> VDISTLPRVKVDLVKPPFVHAHDQVAKTGPRVVEFTMTIEEKKLVIDREGTEIHAMTFNGSVPGPLMVVHENDYVELRLINPDTNTLLHNIDFHAATGALGGGALTQVNPGEETTLRFKATKPGVFVYHCAPEGMVPWHVTSGMNGAIMVLPRDGLKDEKGQPLTYDKIYYVGEQDFYVPKDEAGNYKKYETPGEAYEDAVKAMRTLTPTHIVFNGAVGALTGDHALTAAVGERVLVVHSQANRDTRPHLIGGHGDYVWATGKFRNPPDLDQETWLIPGGTAGAAFYTFRQPGVYAYVNHNLIEAFELGAAGHFKVTGEWNDDLMTSVVKPASM

Copper nitrite reductases (CuNiRs) found in fungi, bacteria and archaea belong to a highly conserved enzyme family that catalyze the one-electron reduction of nitrite to NO [NO2− + e− + 2H+ ⇆ NO + H2O]. The involvement of CuNiRs in two branches of the global nitrogen cycle, denitrification and nitrification, make them of critical environmental importance since N2O is a major by-product of denitrification, which is the third most significant greenhouse gas with a global warming potential 300 times that of CO2.3 The catalytic type 2 Cu centre (T2Cu) of CuNiR is located at the interface of two adjacent monomers and linked to the electron-donating T1Cu centre via a Cys–His bridge. Two invariant active site pocket residues AspCAT and HisCAT are involved in substrate-binding and catalysis and a conserved IleCAT residue provides steric control of ligand binding to the T2Cu. We have undertaken crystallographic studies at a higher temperature of 170 K (normal temperature for synchrotron X-ray data collection is 100 K) at atomic resolution (<1.20 Å) confirming the formation of a side on nitrosyl intermediate during catalysis in crystals and show by DFT calculations that the stability of the {CuNO}10 side-on form is governed by the protonation state of the histidine ligands in the catalytic pocket.

The MSOX series at 170 K, reported here, at atomic resolution is comparable with those determined at other temperatures, reproducing key mechanistic features including the orientation of nitrite and its bidentate mode of binding, changes to occupancy of the gatekeeper and proximal rotamer conformations of AspCAT and the formation of an NO intermediate, demonstrating the presence of side-on NO in crystals of CuNiR during an in situ turnover. The atomic resolution of these crystallographic data sets allowed us to deploy SHELXL for an unrestrained refinement and determine the structural details with sufficient accuracy to underpin the chemistry of the catalytic site during turnover. In dataset 1 (Ds1), clear electron density is apparent for a nitrite molecule bound to the catalytic type 2 Cu site in a highly asymmetric bidentate orientation with Cu–O2 and Cu–O1 (nitrite) bonds 1.88(3) and 2.51 Å, respectively with an occupancy of 0.75 nitrite. The Cu–N (nitrite) distance was 2.42(6) Å.>MEKKLSDAQVALVAAWRKYPDLRESLEEAASILSLIVFQAETLSDQANELANYIRRQGLEEAEGACRNIDIMRAKWVEVCGEVNQHGIRVYGDA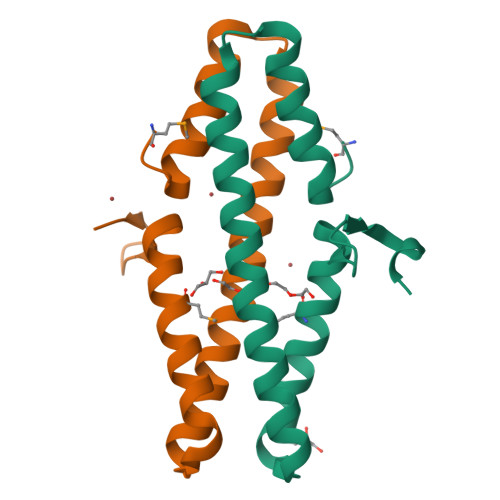IDRDVDLEHHHHHH[3x]> MNPVNATALYISASRLVL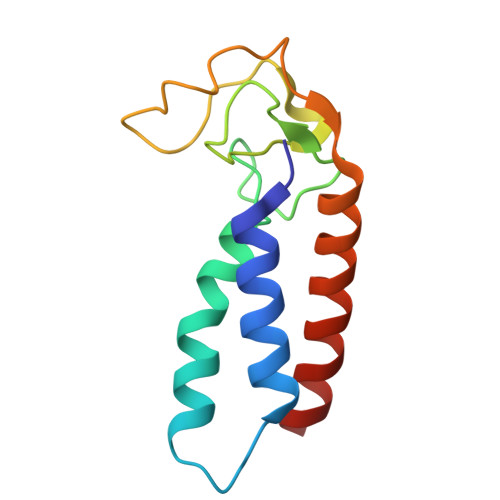NYDPGDPKAFTEINRLLPYFRQSLSCCVCGHLLQDPIAPTNSTCQHYVCKTCKGKKMMMKPSCSWCKDYEQFEENKQLSILVNCYKKLCEYITQTTLA>[30x]AEPNAAT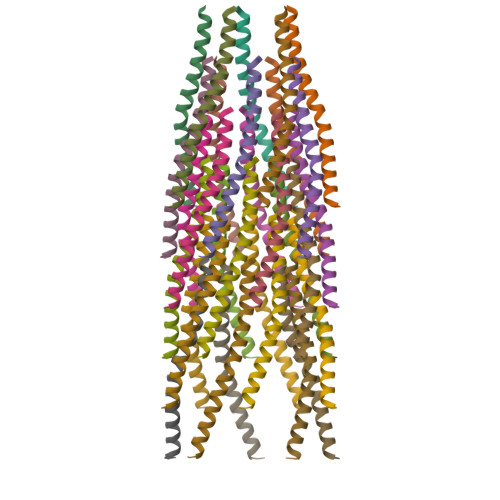NYATEAMDSLKTQAIDLISQTWPVVTTVVVAGLVIRLFKKFSSKAV> ETVPVKLKPGMDGPKVKQWPLTEEKIKALVEICTEMEKEGKISKIGPENPYNTPVFAIKKKDSTKWRKLVDFRELNKRTQDFWEVQLGIPHPAGLKKKKSVTVLDVGDAYFSVPLDEDFRKYTAFTIPSINNETPGIRYQYNVLPQGWKGSPAIFQSSMTKILEPFKKQNPDIVIYQYMDDLYVGSDLEIGQHRTKIEELRQHLLRWGLTTPDKK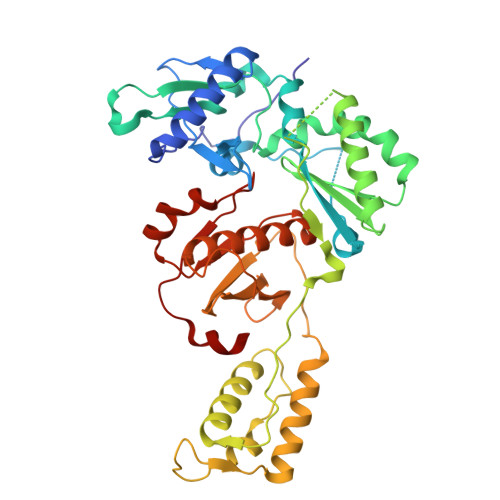HQKEPPFLWMGYELHPDKWTVQPIVLPEKDSWTVNDIQKLVGKLNWASQIYPGIKVRQLSKLLRGTKALTEVIPLTEEAELELAENREILKEPVHGVYYDPSKDLIAEIQKQGQGQWTYQIYQEPFKNLKTGKYARMRGAHTNDVKQLTEAVQKITTESIVIWGKTPKFKLPIQKETWETWWTEYWQATWIPEWEFVNTPPLVKLWYQ N-{(2S,3S)-4-[3-(dimethylamino)-1,2,4-oxadiazol-5-yl]-3-hydroxy-1-phenylbutan-2-yl}-4-(2-methylbutan-2-yl)benzene-1-sulfonamide | C25 H34 N4 O4 S | 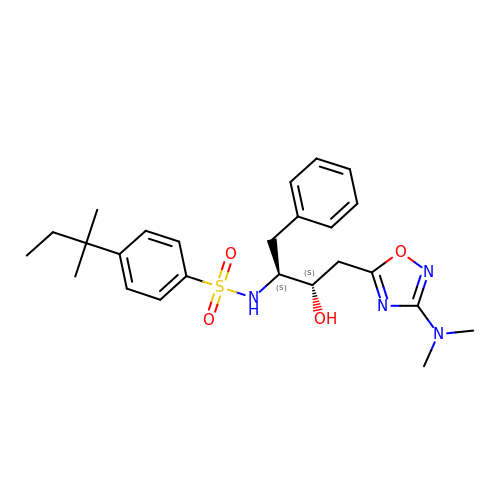MDDQVOFJDJRHHJ-VXKWHMMOSA-N> GPLGSMRRSKADVERYIASV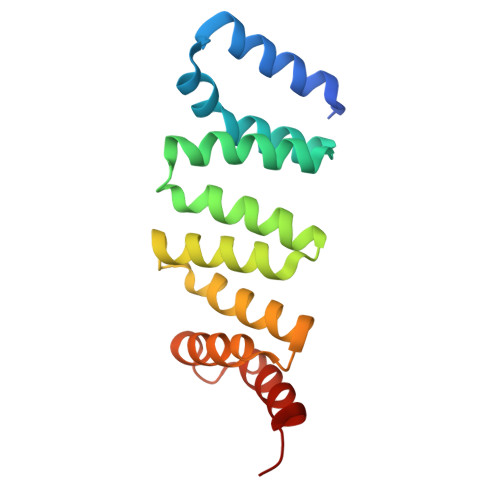QGSTPSPRQKSMKGFYFAKLYYEAKEYDLAKKYICTYINVQERDPKAHRFLGLLYELEENTDKAVECYRRSVELNPTQKDLVLKIAELLCKNDVTDGRAKYWLERAAKLFPGSPAIYKLKEQLLDCEGED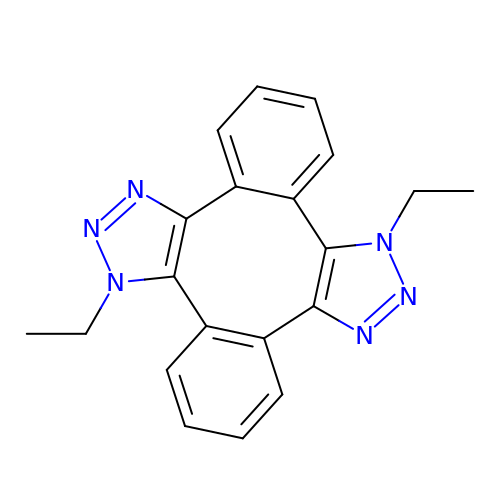1,8-DIETHYL-1,8-DIHYDRODIBENZO[3,4:7,8][1,2,3]TRIAZOLO[4',5':5,6]CYCLOOCTA[1,2-D][1,2,3]TRIAZOLE | C20 H18 N6 | YRZRZRBFIALCLI-MKVCYXFSSA-N>[2x]SLVQFETLIMKIAGRSGLLWYSAYGCYCGWGGH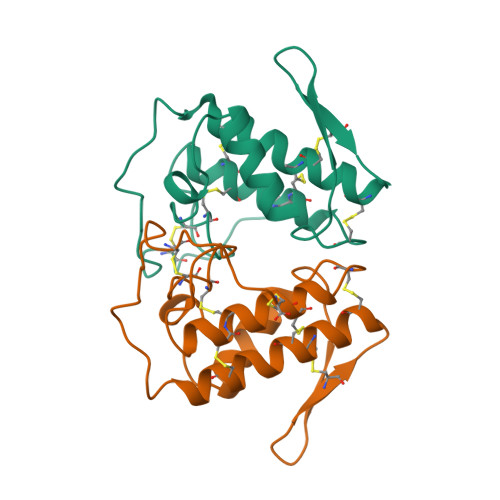GLPQDATDRCCFVHDCCYGKATDCNPKTVSYTYSEENGEIICGGDDPCGTQICECDKAAAICFRDNIPSYDNKYWLFPPKDCREEPEPC>MSVEKIPGYTYGETENRAPFNLEDLKLLKEAVMFTAEDEEYIQKAGEVLEDQVEEILDTWYGFVGSHPHLLYYFTSPDGTPNEKYLAAVRKRFSRWILDTSNRSYDQAWLDYQYEIGLRHHRTKKNQTDNVESVPNIGYRYLVAFIYPITATMKPFLARKGHTPEEVEKMYQAWFKATTLQVALWSYPYVKYGDF[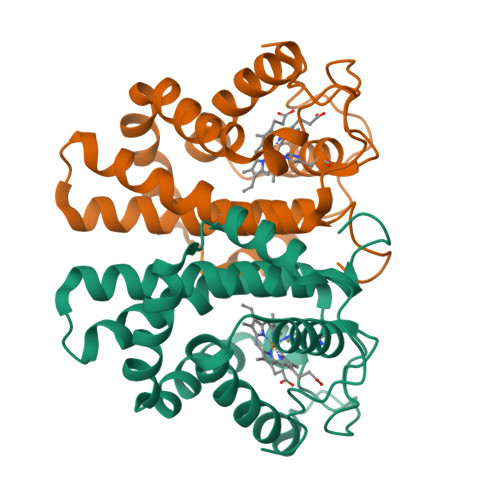8x]(2S)-2-hydroxy-N-[[3-[5-hydroxy-4-(1H-pyrrolo[3,2-c]pyridin-2-yl)pyrazol-1-yl]phenyl]methyl]-3-phenylpropanamide 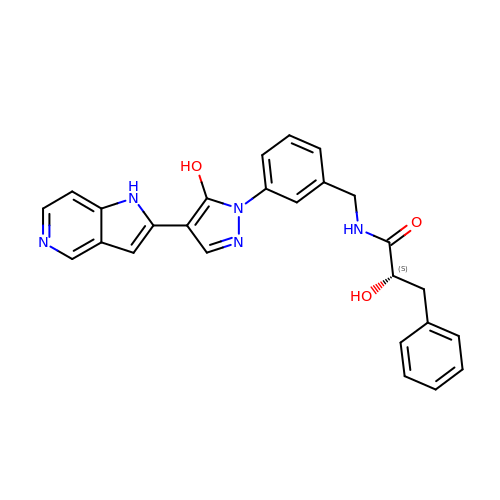| C26 H23 N5 O3 | DVKKUFFDFYCKKJ-DEOSSOPVSA-N>MDQRQKLQHWIHSCLRKADKNKDNKMNFKELKDFLKELNIQVDDGYARKIFRECDHSQTDSLEDEEIETFYKMLTQRAEIDRAFEEAAGSAETLSVERLVTFLQHQQREEEAGPALALSLIERYEPSETAKAQRQMTKDGFLMYLLSADGNAFSLAHRRVYQDMDQPLSHYLVSSSHNTYLLEDQLTGPSSTEAYIRALCKGCRCLELDCWDGPNQEPIIYHGYTFTSKILFCDVLRAIRDYAFKASPYPVILSLENHCSLEQQRVMARHLRAILGPILLDQPLDGVTTSLPSPEQLKGKILLKGKKLGGLLPAGGENGSEATDVSDEVEAAEMEDEAVRSQVQHKPKEDKLKLVPELSDMIIYCKSVHFGGFSSPGTSGQAFYEMASFSESRALRLLQESGNGFVRHNVSCLSRIYPAGWRTDSSNYSPVEMWNGGCQIVALNFQTPGP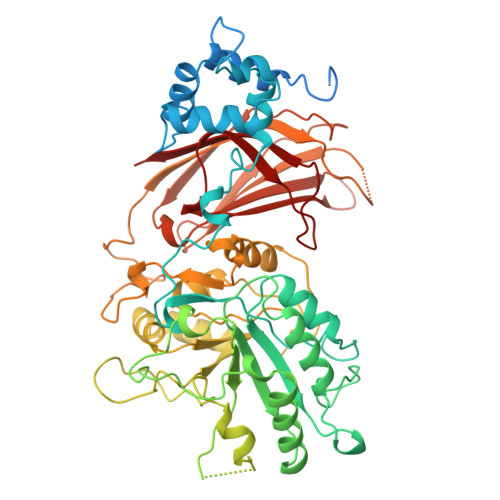EMDVYLGCFQDNGGCGYVLKPAFLRDPNTTFNSRALTQGPWWRPERLRVRIISGQQLPKVNKNKNSIVDPKVIVEIHGVGRDTGSRQTAVITNNGFNPRWDMEFEFEVTVPDLALVRFMVEDYDSSSKNDFIGQSTIPWNSLKQGYRHVHLLSKNGDQHPSATLFVKISIQD[2x]>TPEMPVLENRAAQGDITAPGGARRLTGDQTAALRDSLSDKPAKNIILLIGDGMGDSEITAARNYAEGAGGFFKGIDALPLTGQYTHYALNKKTGKPDYVTDSAASATAWSTGVKTYNGALGVDIHEKDHPTILEMAKAAGLATGNVSTAELQDATPAALVAHVTSRKCYGPSATSEKCPGNALEKGGKGSITEQLLNARADVTLGGGAKTFAETATAGEWQGKTLREQAQARGYQLVSDAASLNSVTEANQQKPLLGLFADGNMPVRWLGPKATYHGNIDKPAVTCTPNPQRNDSVPTLAQMTDKAIELLSKNEKGFFLQVEGASIDKQDQAANPCGQIGETVDLDEAVQRALEFAKKEGNTLVIVTADHAHASQIVAPDTKAPGLT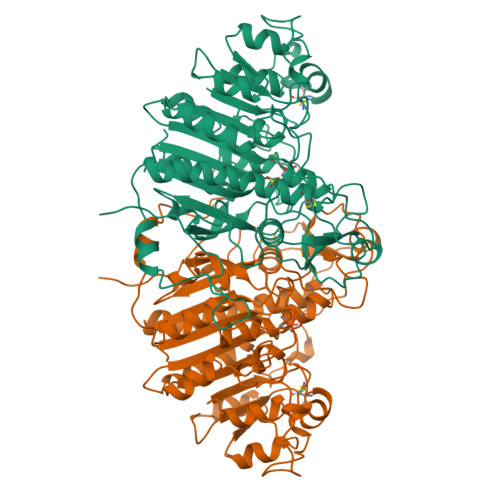QALNTKDGAVMVMSYGNSEEDSQEHTGSQLRIAAYGPHAANVVGLTDQTDLFYTMKAALGLK[2x]>M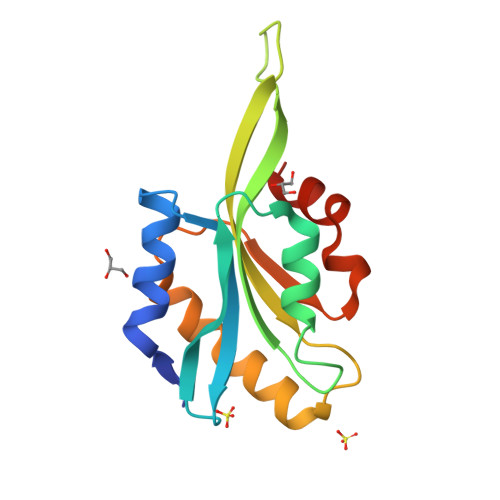ASGVTVSDVCKTTYEEIKKDKKHRYVIFYIRDEKQIDVEVIGDRNAEYDSFLEDIQKGGPGECRYGLFDFEYMHQCQGTSESSKKQKLFLMSWCPDTAKVKKKMLYSSSFDALKKSLVGVQKYIQATDLSEASREAVEEKLRATDRQ[2x]>[2x]MSIVVKNNIHWVGQRDWEVRDFHGTEYKTLRGSSYNSYLIREEKNVLIDTVDHKFSREFVQNLRNEIDLADIDYIVINHAEEDHAGALTELMAQIPDTPIYCTANAIDSINGHHHHPEWNFNVVKTGDTLDIGNGKQLIFVETPMLHWPDSMMTYLTGDAVLFSNDAFGQHYCDEHLFNDEVDQTELFEQCQRYYANILTPFSRLVTPKITEILGFNLPVDMI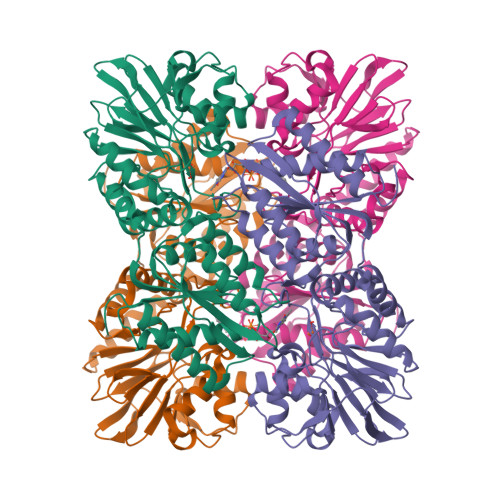ATSHGVVWRDNPTQIVELYLKWAADYQEDRITIFYDTMYNNTRMMADAIAQGIAETDPRVAVKIFNVARSDKNEILTNVFRSKGVLVGTSTMNNVMMPKIAGLVEEMTGLRFRNKRASAFGSHGWSGGAVDRLSTRLQDAGFEMSLSLKAKWRPDQDALKLCREHGREIARQWALAPLPQSTVNTVVKE>MGNKYRVRKNVLHLTDTEKRDFVRTVLILKEKGIYDRYIAWHGAAGKFHTPPGSDRNAAHMSSAFLPWHREYLLRFERDLQSINPEVTLPYWEWETDAQMQDPSQSQIWSADFMGGNGNPIKDFIVDTGPFAAGRWTTIDEQGNPSGGLKRNFGATKEAPTLPTRDDVLNALKITQYDTPPWDMTSQNSFRNQLEGFINGPQLHNR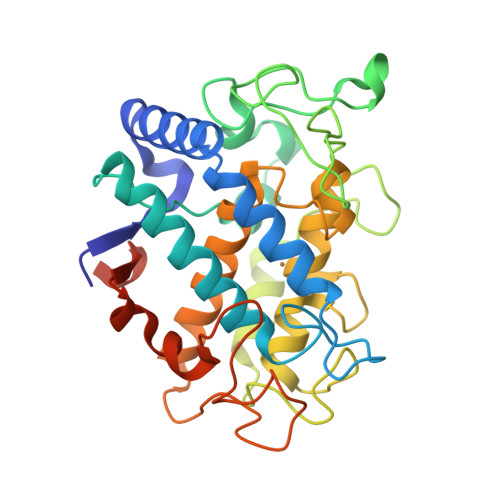VHRWVGGQMGVFPTAPNDPVFFLHHANVDRIWAVWQIIHRNQNYQPMKNGPFGQNFRDPMYPWNTTPEDVMNHRKLGYVYDIELRKSKRSSHHHHHH[2x]>MALSKSMHARNRYKDKPPDFAYLASKYPDFKQHVQINLNGRVSLNFKDPEAVRALTCTLLREDFGLSIDIPLERLIPTVPLRLNYIHWVEDLIGHQDSDKSTLRRGIDIGTGASCIYPLLGA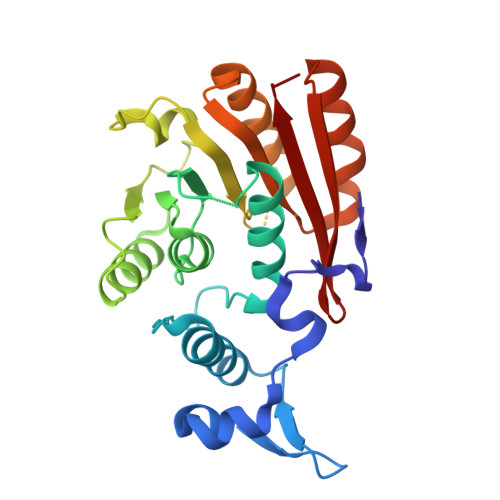TLNGWYFLATEVDDMCFNYAKKNVEQNNLSDLIKVVKVPQKTLLMDALKEESEIIYDFCMCNPPFFANQLEAKGVNSRNPRRPPPSSVNTGGITEIMAEGGELEFVKRIIHDSLQLKKRLRWYSCMLGKKCSLAPLKEELRIQGVPKVTYTEFCQGRTMRWALAWSFYD[2x]> MSETTERTVLGEYNLFSRKIEEILKQKNVSYVS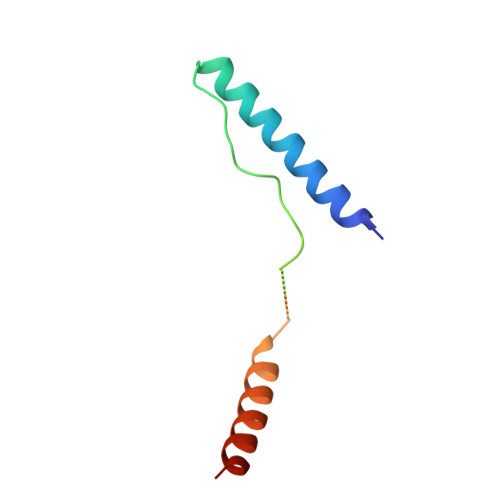TVSTPIFSTQEKMKRLSEFIYSKTSKAGVQEFVDGLHEKLNTIIIKASAK> APVWGCASTRGRSAEMEDASAAVPRFADVPVRLLASRRDLDALGLDADALRLPAHLFGVFDGHGGAEVANYCRERIHVVLSAALARLGKNLGEMGEVDMKEHWDDVFTKCFQRVDDEVSGRVTRVVNGGGEVRSEPVTAENVGSTAVVALVCSSHVVVANCGDSRIVLCRGKEPVALSIDHKPDRKDE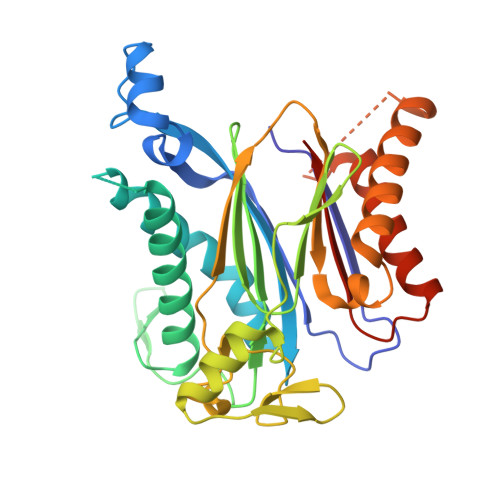RARIEAQGGKVIQWNGYRVSGILAMSRSIGDRYLKPFVIPKPEVMVVPRAKDDDCLILASDGLWDVVSNEEACKVARRQILLWHKNNGAASPLSDEGEGSTDPAAQAAADYLMRLALKKGSEDNITVIVVDLKPRKKLKN> MEANGLGPQGFPELKNDTFLRAAWGEETDYTPVWCMRQAGRYLPEFRETRAAQDFFSTCRSPEACCELTLQPLRRFPLDAAIIFSEILVVPQALGMEVTMVPGKGPSFPEPLREEQDLERLRDPEVVASELGYVFQAITLTRQRLAGRVPLIGFAGAPWTLMTYMVEGGGSSTMAQAKRWLYQRPQASHQLLRILTDALVPYLVGQVVAGAQALQLFESHAGHLGPQLFNKFALPYIRDVAKQVKARLREAGLAPVPMIIFAKDGHFALEELAQAGYEVVGLDWTVAPKKARECVGKT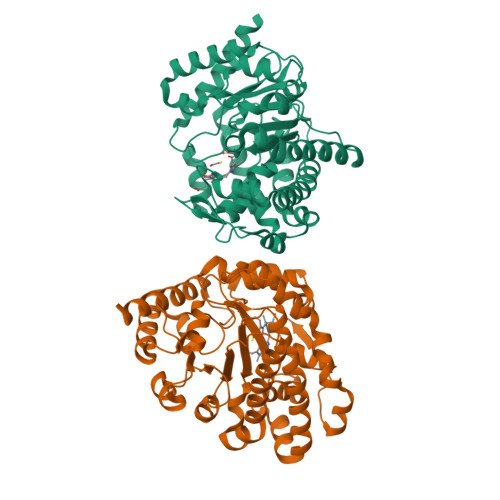VTLQGNLDPCALYASEEEIGQLVKQMLDDFGPHRYIANLGHGLYPDMDPEHVGAFVDAVHKHSRLLRQN> CGRKRRQTSMTDFYHS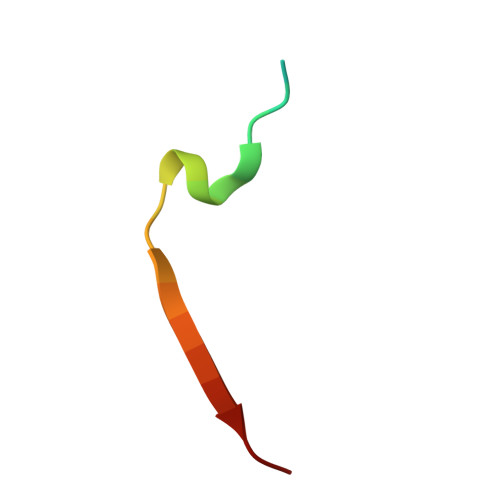KRRLIFS> MERIVIVGGGLAASRTCEQLRSRGYEGELVMLCAEPHPPYDRPPLSKAALLEEEHDSTFPTDYAQLSVDVRLGVAATGLVPDARTVQTTDGELSYDALVIATGASPIRLPGPGRQFTVRTVEDAAQLRAELKPGQRVVLVGASWISAEVATAALRRGCSVTCIEAGPAPLSAALGADVGQRFLPWWSEVDLRLDTGVAEVTETGVQLANGEQVDADVVVTGIGVRPAVDWLSGSGIALDTGVVV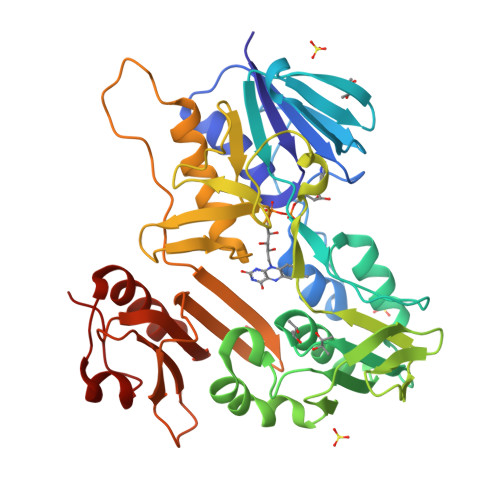DEHLRTSLPGIYALGDVAVRWSPRWNTRIRVEHWDDAREAARTLAGVLLHDPSSQDPLPVHDPVPYFWSDQFGHKIQYVGHHSPEDTLVIRGDGTPQWAAAWVDAEGRLTAHLSIDAPRLMIDARMAIAAGARPDEAALRDPQAKLAPP>GHMSQEEKLP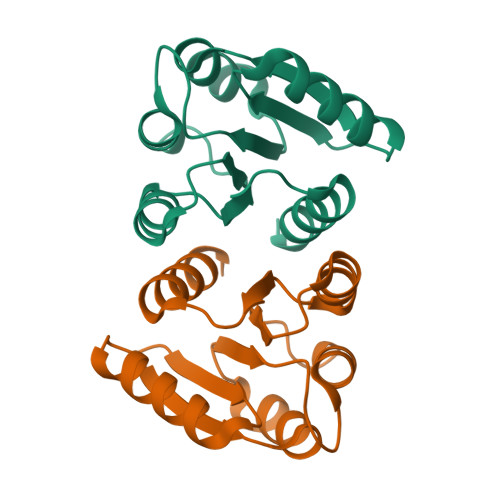KILIVEDDERLARLTQEYLIRNGLEVGVETDGNRAIRRIISEQPDLVVLDVMLPGADGLTVCREVRPHYHQPILMLTARTEDMDQVLGLEMGADDYVAKPVQPRVLLARIRALLRRTDKTVE[2x]> RCCHPQCGMA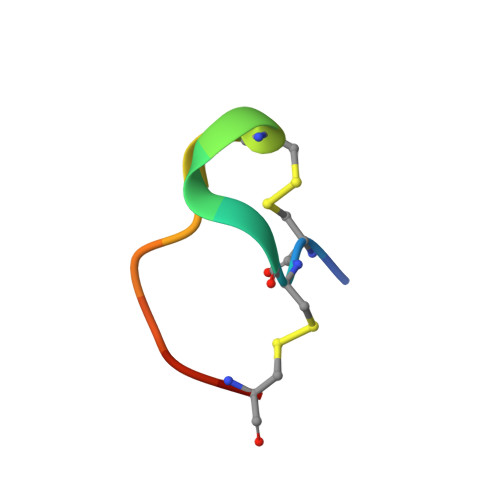EECR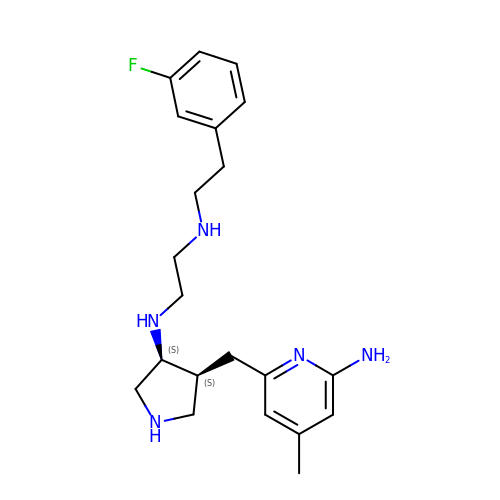N-{(3S,4S)-4-[(6-amino-4-methylpyridin-2-yl)methyl]pyrrolidin-3-yl}-N'-[2-(3-fluorophenyl)ethyl]ethane-1,2-diamine | C21 H30 F N5 | PUOKPLCASUFBAN-FXAWDEMLSA-N>[3x]VINTFDGVADYLQTYHKLPDNY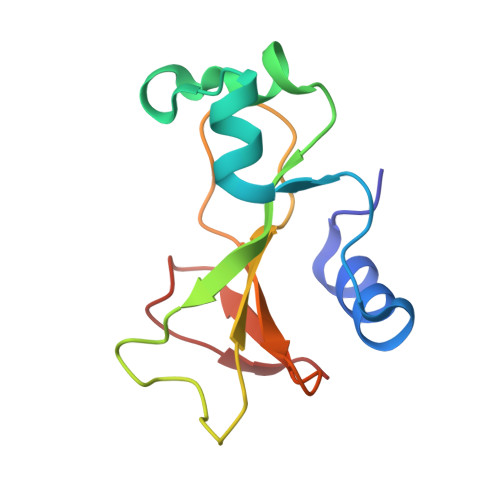ITKSEAQALGWVASKGNLADVAPGKSIGGDIFSNREGKLPGKSGRTWREADINYTSGFRNSDRILYSSDWLIYKTTDHYQTFTKIR>MSAEVETSEGVDESEKKNSGALEKENQMRMADLSELLKEGTKEAHDRAENTQFVKDFLKGNIKKELFKLATTALYFTYSALEEEMERNKDHPAFAPLYFPMELHRKEALTKDMEYFFGENWEEQVQAPKAAQKYVERIHYIGQNEPELLVAHAYTRYMGDLSGGQVLKKVAQRALKLPSTGEGTQFYLFENVDNAQQFKQLYRARMNALDLNMKTKERIVEEANKAFEYNMQIFNELDQAGSTLARETLEDGFPVHDGKGDMRK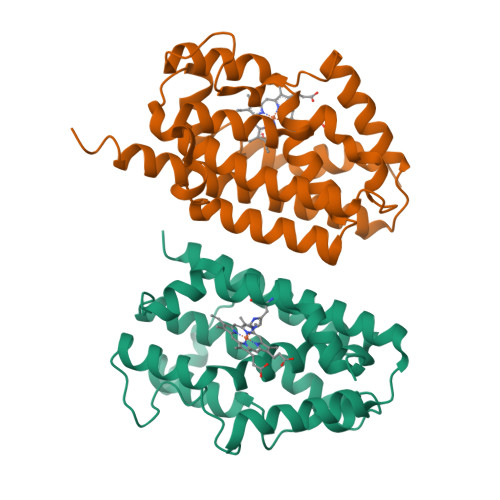[2x]2,4-dinitrophenyl 2-deoxy-2-fluoro-beta-D-mannopyranoside 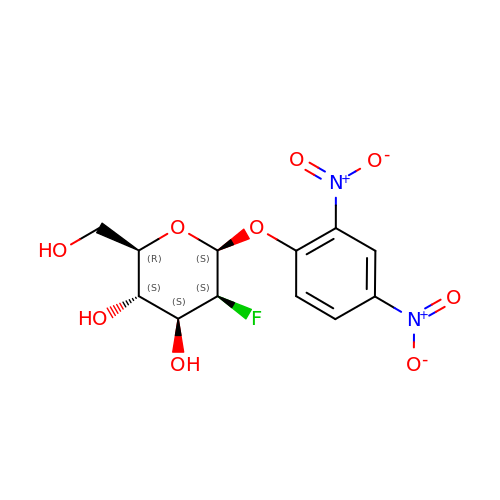| C12 H13 F N2 O9 | UFSBFVZQJZMIOU-IYKVGLELSA-N>MDVSLPCIKIQVQTRYIEEQSNPEYQRFVFAYLITIKNLSSQTVQLMSRRWLITDADGKQT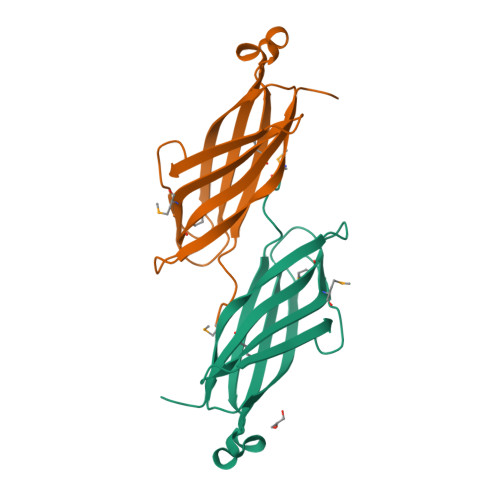VVEGDGVVGEQPRIKANDEYTYSSGTALDTPVGVMQGQYLMIDEQGESFTVEIEPFRLAVPHVLN[2x]The α1-acid glycoprotein (AGP) is an abundant blood plasma protein with important immunomodulatory functions coupled to endogenous and exogenous ligand-binding properties. Its affinity for many drug-like structures, however, means AGP can have a significant effect on the pharmokinetics and pharmacodynamics of numerous small molecule therapeutics. Human plasma lipocalins present as two variants known as AGP1 and AGP2 (or F1/F2/S and A forms, respectively). The AGP2 structure has an archetypal eight-stranded antiparallel β-barrel structure that is characteristic of AGP and lipocalin folds.

Cocrystallization of UCN-01 with AGP2 yielded crystals diffracting to 1.82 Å representing the highest resolution achieved for an AGP2 complex to date. UCN-01 makes multiple contacts with the binding pocket and sits in a plane almost perpendicular to the axis of the β-barrel. Several aromatic residues line the binding pocket including Tyr37, Phe49, Phe51, His97, Phe112, and Tyr127 and form interactions with UCN-01 which is principally comprised of an extended aromatic ring system. Phe112 forms a CH-π interaction with the central benzene ring of UCN-01 and the Tyr127 hydroxyl group H-bonds to indole nitrogen N2. Glu64 and Arg90 sit above the plane of UCN-01 and form a salt-bridge connecting β-strands C and E. This carboxylate – guanidinium group interaction lies perpendicular to the UCN-01 aromatic system allowing the formation of a hydrogen bond from the lactam ring 7R-OH to Glu64 and a cation-π interaction with Arg90. Tyr37 appears to form a parallel VdW interaction with one face of the oxy-bridged seven membered ring of UCN-01. Comparison with all four complexes shows that Phe112 is rotated toward the ligand plane of aromaticity in the case of CPZ and UCN-01, whereas it lies flat and is more restricted in the AMT and DSP complexes. The structure reveals that the hydroxyl group of UCN-01 is important and is oriented toward Glu64, forming a hydrogen bond and indirectly assisting with orienting Arg90. However, the reversal of the stereochemistry at C7 not only breaks this hydrogen bonding, but is likely to invoke a clash with Phe49 and a further shift from the optimal binding pose. The addition of UCN-01 to AGP2 resulted in a significant increase in the melting temperature shifting by 13.7 °C from 61.9 °C to 75.6 °C, again indicative of high affinity binding of UCN-01 and thermal stabilization of the truncated form.

> MAHHHHHHSSGLEVLFQGPQIPLCANLVPVPITNATLDRITGKWFYIASAFRNEEYNKSVQEIQATFFYFTPNKTEDTIFLREYQTRQNQCFYNSSYLNVQRENGTVSRYEGGREHVAHLLFLRDTKTLMFGSYLDDEKNWGLSFYADKPETTKEQLGEFYEALDCLRIPRSDVMYTDWKKDKCEPLEKQH>MKNPLTLSKEEEVLQNLQSFSAHFKQVLKNEKPLVYYGVLKAKAPNWALWVYEKPLKKEIYMNDKEVVVYEPNLFQATITPLKDKTDFFTILKQLKKQTDGSFKTTINKTTYRLVFKDGKPFSLEFKDDMNNLVTITFSQAEINPKIPNEIFVFNPKDENIDI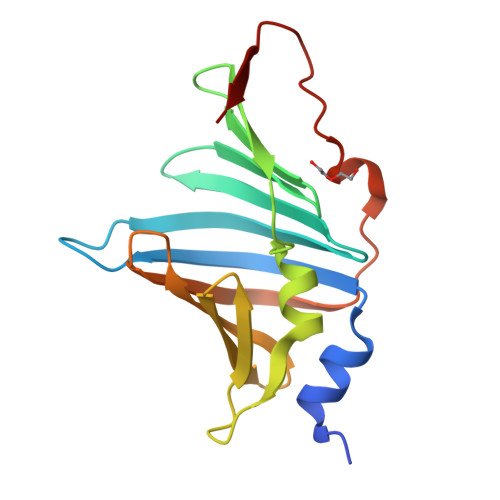VRQ[2x]> MLRDLFDRAVVLSHYIHNLSSEMFSEFDKRYTHGRGFITKAINSCHTSSLAT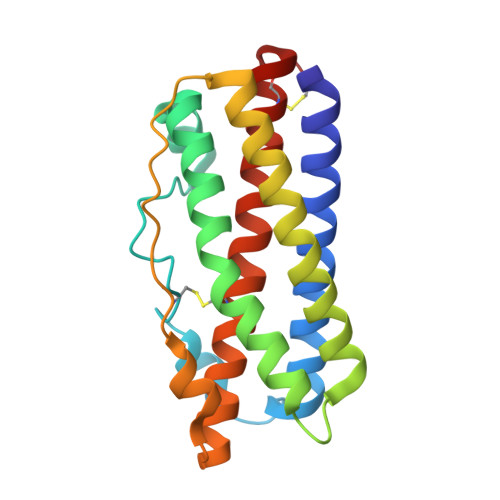PEDKEQAQQMNQKDFLSLIVSILRSWNEPLYHLVTEVRGMQEAPEAILSKAVEIEEQTKRLLERMELIVSQVHPETKENEIYPVWSGLPSLQMADEESRLSAYYNLLHCLRRDSHKIDNYLKLLKCRIIHNNNC> MGSSHHHHHHSQDPMSLIKKKNKDIRIIPLGGVGEIAKNMYIVEVDDEMFMLDAGLMFPEDEMLGVDIVIPDIQYVIENKERLKGIFLTAGHEHAIGAVSYVLEQIDAPVYGSKLTIALVKEAMKARNIKKKVRYYTVNHDSIMRFKNVNVSFFNTTHSIPDSLGVCIHTSYGSIVYTGEFKFDQSLHGHYAPDLKRMAEIGDEGVFALISDSTEAEKPGYNTPENIIEHHMYDAFAKVKGRLIVSCYASNFVRIQQVLNIASQLNRKVSFLGRSLESSFNIARKMGYFDIPKDLLIPINEVENYPKNEVIIIATGMQGEPVEALSQMARKKHKIMNIEEGDSIFLAITASANMEVIIADTLNELVRAGAHIIPNNKKIHASSHGCMEELKMMLNIMKPEYFVPVQGEFKMQIAHAKLAAETGVAPEKIFLVEKGDVISYNGKDMILNEKVQSGNILIDGIGVGDVGNIVLRDRHLLAEDG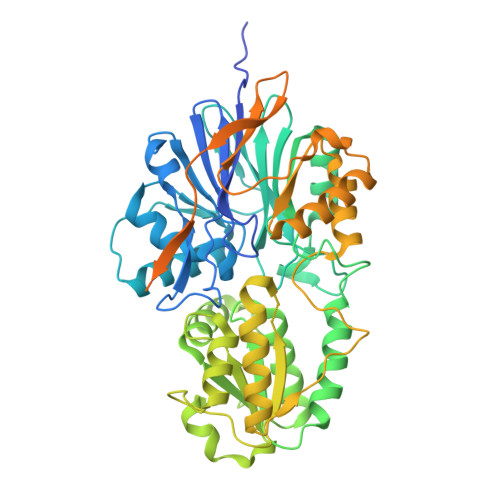IFIAVVTLDPKNRRIAAGPEIQSRGFVYVRESEELLKEAEEKVRKIVEEGLQEKRIEWSEIKQNMRDQISKLLFESTKRRPMIIPVISEI>MRGSHHHHHHGSACELMQILLANPRGFCAGVDRAISIVENALAIYGAPIYVRHEVVHNRYVVDSLRERGAIFIEQISEVPDGAILIFSAHGVSQAVRNEAKSRDLTVFDATCPLVTKVHMEVARASRRGEESILIGHAGHPEVEGTMGQYSNPEGGMYLVESPDDVWKLTVKNEEKLSFMTQTTLSVDDTSDVIDALRKRFPKIVGPRKDDICYATTNRQEAVRALAEQAEVVLVVGSKNSSNSNRLAELAQRMGKRAFLIDDAKDIQEEWVKEVKCVGVTAGASAPDILVQNVVARLQQLGGGEAIPL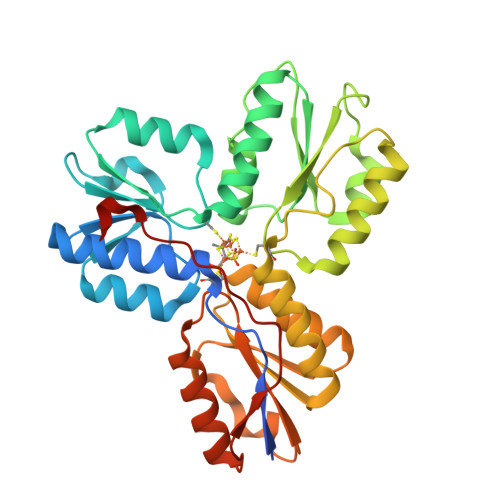EGREENIVFEVPKELRVDIREVD[2x]> HKCDITLQEIIKTLNSLTEQKTLCTELTVTDIFAASKNTTEKETFCRAATVLRQFYSHHEKDTRCLGATAQQFHRHKQLIRDLKRLDRNLWGLAGLNSCPVKEANQSTLENFLER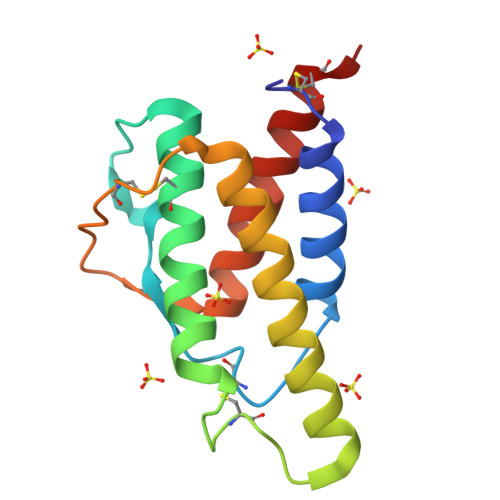LKTIMREKYSKCSS>MALGTSGVKIHPNGNSNQLGVQLENVKLTSLFKKLDKRCSLASWIKENIKKKECCFYVEDGREGICKCGYPKVQHCDEAIKPEDYMGEQWDKHRHVRETPTDAFGDISFGGLGQKTGKYVRVSSDTSCENLYQLMTEQWKLRSPNLLISVTGGAKNFYIKTHLKDKFRRGLIKVAQTTGAWILTGGTHAGVMKHVGMAVRDYTLSSGSMEGQIVVIGVAPWGVIHNRSTLIHPEGRFPAYYSLDEQGQGRLSCLDINHTHFLLVDDGTQGHYGVEIELRARLEKLISKLSLGNRESGVTIPVVCVVLDGGPGTLNTIYNSMLNHTPCVVLEGSGRLADVIAHVASVPVSKVTMALINRLLKRFFMQEYKNFTELQIIEWTKKIQDILRMPHLLTVFRIDEDKNYDVDVAILQALLKASRSDEHAGRHCWERQLELAVAWNRVDIAESEIFTEESQWTSSDLHPAMFSALVGDKPEFVRLLLENGVCVREFLEREETLCELYSHLPSCFFLRKLAKRVQGGKMRRGQEPLPGSRKVCLSHVSEEVRHLLGSFTQPLYIASRYKPTKDDVRLKVPSKGALDLPCSGEEWSADTVWDPGRDLFLWAVVQNNRELAEIGWEQCRDCIAAALAASKILRKLAQESGEDDSEEATEMLELANHYEKQAIGVFSECHSWDAQRAQKLLIRISPSWGRSTCLWLALEAHDKSFIAHSGVQALLTQIWCGELSVDNPHWKVLLCMIFFPLIYTGFLTFRRDEDIQRQAERTEQQKLAMESVFAGQSDGKIKRHLRGFSQKSELKPLNCSSRLMSFLKSPQVKFYWNIASYFGFLWLFAVVLMIDFQTSPSWRELLLYVWLTSLVCEEIRQLYHDFDGSGFRRKAKMYIKDLWNILDVLSIVLFIAGLICRLQASDTVFYIGKVILCIDFIIFCLRLMAIFSISRTLGPKIIIVRRMMLDLFFFMFLLSIWVVAYGVAKQGILIENEERLNWIIRGAVYEPYITIFGNFPTNIDNTLFDISSCSVNASDPLKPKCPMLNADNTPVFPEWLTIMMLCVYLLFANILLLNLLIAIFNYTFQEVQDNTDTIWKFQRYELIKEYHSRPALPPPFILLSHLILFIRGVFLRDLPQRHKNFRQELEQTEEEELLSWEAYMKDNYLASTRQDESQSVEHRIHDTAEKVGAMSELLEREQEMVXXXXXXXXXXXXXXXXXXXXXXDEEAPHMFARQLQYPDSTVRRFPVPEEKVSWEVNFSPYQPPVYNQQDSSESDTSALDKHRNPGGRTGIRGKGALNTLGPNHILHPIFTRWRDAEHKVLEFLAVWEDAEKRWALLGGPAQPDEPLAQVLERILGKKLNEKTKTLLKAGEEVYKGYVDDSRNTDNAWVETSIITLHCDKNTPLMADLNHMVESSLSSHQPLQWREVSSDACRCSYQREALRQIAHHHNTYFSNSLEVLFQGPDYKDDDDKAHHHHHHHHHH[4x]

TRPM2 is a calcium-permeable nonselective cation channel that is widely expressed in the nervous, immune, and endocrine systems, and plays a crucial role in warmth and redox-dependent signaling. Extensive electrophysiological studies have shown that activation of TRPM2 by ROS is caused by an increase of intracellular ADP-ribose (ADPR), a TRPM2 agonist, and that both ADPR and Ca2+ are required for channel activation. Our TRPM2DR channel forms a homo-tetramer. Similar to the previously reported TRPM2, TRPM4, and TRPM8 structures, each TRPM2DR protomer contains an N-terminal region composed of MHR1 to MHR4, a transmembrane channel region, and a C-terminal region.

We prepared the TRPM2DR_Apo according to the method published for the TRPM2closed structure. In brief, the protein was purified in Ca2+-free buffer and incubated with 1 mM EDTA before sample vitrification (see “Methods”). Following Bayesian polishing, the shiny particles were subjected to a final round of 3D auto-refinement with C1 symmetry. This 3D reconstruction exhibited an overall apparent four-fold (C4) symmetry, but closer visual inspection revealed a slight deviation of the C4 symmetry in the TMD. We therefore chose to proceed with the refinement in a conservative manner and refined the shiny particles with both C2 and C4 symmetry imposed in parallel and determined the reconstructions to ~4.5 Å and ~4.3 Å resolution, respectively. Our TRPM2DR_Apo structure with imposed C4 symmetry (referred to as TRPM2DR_Apo-C4) resembles the published four-fold symmetric TRPM2closed structure across different layers of the channel. We determined the TRPM2 structure in the apo conformation (TRPM2DR_Apo-C4), which resembles the published four-fold symmetric TRPM2closed structure, although upon further processing we observed a slight deviation from C4 symmetry in the TMD (TRPM2DR_Apo-pseudo C4). Due to the lower resolution of our TRPM2DR_Apo structures, the published TRPM2closed structure was utilized for our detailed structural analyses of ligand-induced conformational changes.>[4x]AEAGITGTWYNQLGSTFIVTAGADGALTGTAESAVGNAESRYVLTGRYDSAPATDGSGTALGWTVAWKNNYRNAHSATTWSGQYVGGAEARINTQWLLTSGTT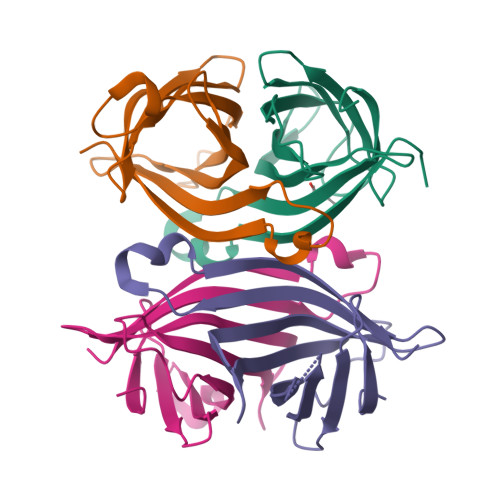EANAWKSTLVGHDTFTKVKPSAAS>GPDSMPRGADQENMLKISGYPGMLNTFGIAQLLTPYRVNGITITGAQSAVVAL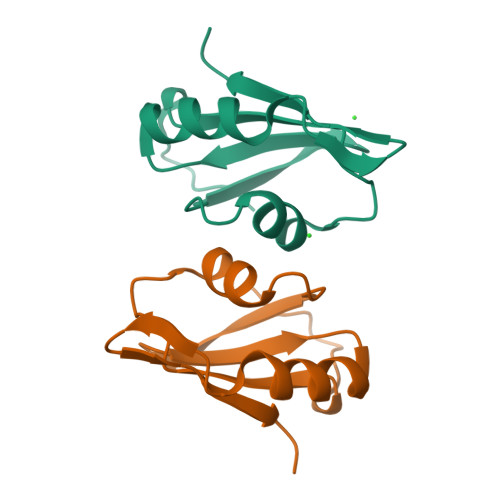ENKFQVYQAVQDFNGKKLDRNHKLQVSSLVV[2x]>MGSSHHHHHHSSGETVRFQGHMDVVDPDIFNRDPRDHYDLLQRLGGGTYGEVFKARDKVSGDLVALKMVKMEPDDDVSTLQKEILILKTCRHANIVAYHGSYLWLQKLWICMEFCGAGSLQDIYQVTGSLSELQISYVCREVLQGLAYLHSQKKIHRDIKGANILINDAGEVRLADFGISAQIGATLARRLSFIGTPYWMAPEVAAVALKGGYNELCDIWSLGITAIELAELQPP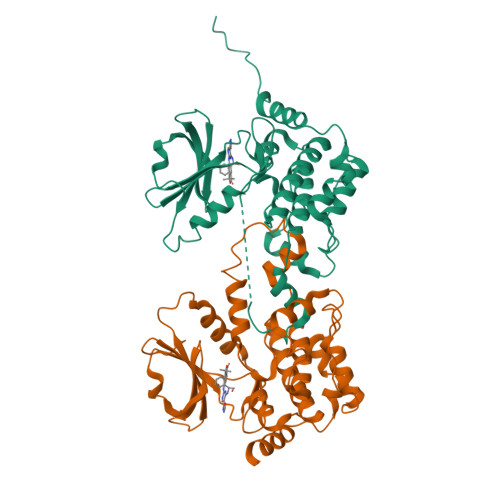LFDVHPDRVLELMTKSGYQPPRLKEKGKWSAAFHNFIKVTLTKSPKKRPSATKMLSHQLVSQPGLNRGLILDLLDKLKNPGKGPSIGDIEDEEPELPPAIPRRIR[2x]> NAVESTLRRVAKDLTGLRQRWALVGGFAVSARSEPRFTRDVDIVVAVANDDAAESLVRQLLTQQYHLLASVEQDAARRLAAVRLGATADTAANVVVDLLFASCGIEPEIAEAAEEIEILPDLVAPVATTAHLIAMKLLARDDDRRPQDRSDLRALVDAASPQDIQDARKAIELITLRGFHRDRD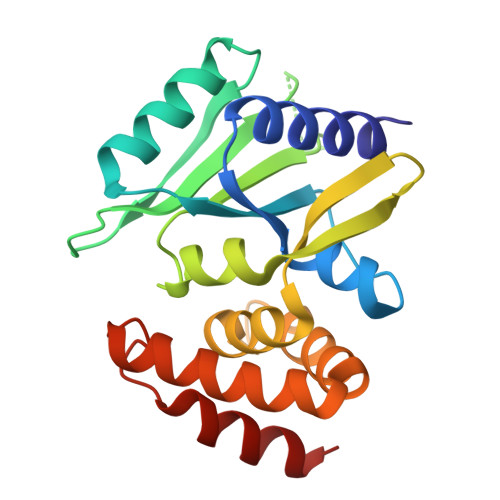LAAEWTRLAAKW>GEFSGPPVERCGVLSKWTNYIHGWQDRWVVLKNNALSYYKSEDETEYGCRGSICLSKAVITPHDFDECRFDISVNDSVWYLRAQDPDHRQQWIDAIEQHKTESGY[2x]

While vesicular trafficking is responsible for the pool of ceramide used for glucosylceramide synthesis, the delivery of ceramide from ER to Golgi for SM synthesis is carried out by a cytosolic lipid transfer protein, the ceramide transfer protein (CERT). The N terminal pleckstrin homology (PH) domain is responsible for its localization to the Golgi by binding to phosphatidylinositol-4-phosphate (PtdIns(4)P) that are enriched in the Golgi membrane. While the START domain alone bears high ceramide transfer activity in vitro, inside the cell, PH domain binding to PtdIns(4)P is essential for CERT function. In this paper, we report a crystal structure of the CERT PH domain and associated biochemical characterization in an effort to understand the structural basis of PH domain mediated CERT localization to the Golgi.

Crystals of the human CERT PH domain spanning residues 20–122 were obtained using ammonium sulfate as a precipitant. The final structure was refined to 1.75 Å resolution. It contains a curved and twisted β-sandwich that is capped by the C terminal α-helix at one open end. Opposite to the capping helix, the other open end of the β-sandwich contains a bound sulfate, which likely originated from the crystallization solution that contained 1.0 M ammonium sulfate. The sulfate forms hydrogen bonds with residues K32, R43, Y54 and R66, all of which are highly conserved among many PH domains and involved in interactions with the PIP ligand. Nuclear magnetic resonance (NMR) studies show sulfate binding mimics 1,2-dihexanoyl (diC6)-PtdIns(4)P binding to the CERT PH domain, thus the sulfate bound crystal structure likely captures the major features of the PtdIns(4)P bound state. The two copies of CERT PH molecules in the asymmetric unit have distinct conformations in the β3–β4 loop. In molecule B, a major portion of this loop points outward and residue R66 from this region is hydrogen bonded with the bound sulfate. In molecule A, the β3–β4 loop points downward and K56 replaces R66 to interact with the sulfate. Structure B likely represents the major conformation while structure A a minor one.> PLQEMLAAPSSFKKSHVLSVTQFTRADLHLLFQIAQEMRLGVQREGVLDILRGKVLCTLFYEPSTRTSASFDAAMQRLGGRTIPIQTSTSSVQKGETLQDTLRTLACYSDAIVLRHPDEKCVDVAKKYCPVPVINGGNGSKEHPTQAFLDLFTIREELGTMQGLTITFVGDLLYGRPVHSLVYLLRHYQVKVQLVSPKALRLPPAVRQQLVDAGQLLCESEALTPEILGRTDVLYCTRVQKERFPSLAEFEAVKDSYRIDYSTLKYAKPTTVVMHPLPRNEEVAEEVDFDQR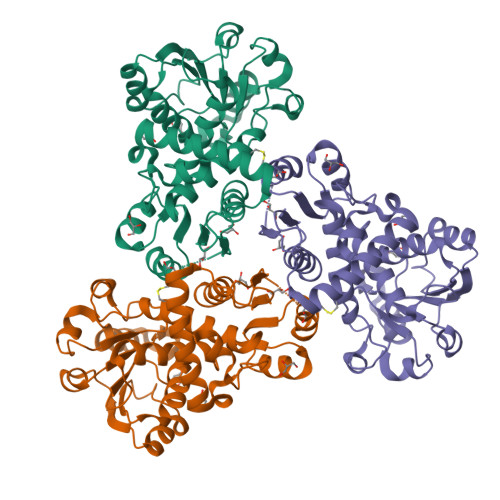AAYFRQMCYGLYCRMALLALVMS Tripartite efflux pumps are essential for Gram-negative bacteria to expel a wide range of toxic compounds, including antibiotics, across their dual-membrane cell envelope. Among these systems, the AcrAB–TolC complex of *Escherichia coli* is one of the most thoroughly studied. It comprises the inner membrane RND (Resistance–Nodulation– Division) transporter AcrB, the periplasmic membrane fusion protein AcrA, and the outer membrane channel TolC. Structural analysis reveals that YbjP, a previously uncharacterized lipoprotein, binds TolC in a 3:3 stoichiometry, bridging its protomers at the equatorial domain.

Cryo-EM density reveals six AcrA molecules beneath each TolC trimer ([Fig fig2]), yielding a 3:6:3 stoichiometry for TolC:AcrA:AcrB. AcrA therefore forms an elongated hexamer that bridges TolC and AcrB. The trimeric TolC, which contains six HTH motifs due to internal repeats (TolC repeat 1/2), engages the AcrA hexamer via quasi-equivalent binding: adjacent AcrA and AcrA* protomers interact differentially with the intra- and inter-protomer grooves of TolC, respectively ([Fig fig2]). Upon engagement with AcrA’s α-helical hairpin domain, TolC helices rotate outward in a left-handed (counterclockwise) manner to open the channel, and enables small-molecule substrates to be exported through the fully assembled complex. A comparative structural analysis of TolC in its closed and open states reveals a striking iris-like dilation mechanism at the periplasmic entrance that facilitates transition to the fully open conformation ([Fig fig3]). Throughout this conformational transition, the transmembrane β-barrel and α-helical barrel domains maintain remarkable structural rigidity, whereas the coiled-coil helices undergo dramatic rearrangement. These helices pivot around the equatorial domain, undergoing a 27° rigid-body superhelical rotation ([Fig fig3]), which constitutes a major structural rearrangement. Notably, YbjP remains stably association with TolC in both conformational states – the closed resting state and the open activated state ([Fig fig3]). This persistent interaction suggests that YbjP serves as a structural scaffold: anchoring TolC in the outer membrane, accommodating conformational changes during activation, and functionally compensating for TolC’s lack of intrinsic lipidation.

>[6x]MNKNRGFTPLAVVLMLSGSLALTGCDDKQAQQGGQQMPAVGVVTVKTEPLQITTELPGRTSAYRIAEVRPQVSGIILKRNFKEGSDIEAGVSLYQIDPATYQATYDSAKGDLAKAQAAANIAQLTVNRYQKLLGTQYISKQEYDQALADAQQANAAVTAAKAAVETARINLAYTKVTSPISGRIGKSNVTEGALVQNGQATALATVQQLDPIYVDVTQSSNDFLRLKQELANGTLKQENGKAKVSLITSDGIKFPQDGTLEFSDVTVDQTTGSITLRAIFPNPDHTLLPGMFVRARLEEGLNPNAILVPQQGVTRTPRGDATVLVVGADDKVETRPIVASQAIGDKWLVTEGLKAGDRVVISGLQKVRPGVQVKAQEVTADNNQQAASGAQPEQSKS;>MKKLLPILIGLSLSGFSSLSQAENLMQVYQQARLSNPELRKSAADRDAAFEKINEARSPLLPQLGLGADYTYSNGYRDANGINSNATSASLQLTQSIFDMSKWRALTLQEKAAGIQDVTYQTDQQTLILNTATAYFNVLNAIDVLSYTQAQKEAIYRQLDQTTQRFNVGLVAITDVQNARAQYDTVLANEVTARNNLDNAVEQLRQITGNYYPELAALNVENFKTDKPQPVNALLKEAEKRNLSLLQARLSQDLAREQIRQAQDGHLPTLDLTASTGISDTSYSGSKTRGAAGTQYDDSNMGQNKVGLSFSLPIYQGGMVNSQVKQAQYNFVGASEQLESAHRSVVQTVRSSFNNINASISSINAYKQAVVSAQSSLDAMEAGYSVGTRTIVDVLDATTTLYNAKQELANARYNYLINQLNIKSALGTLNEQDLLALNNALSKPVSTNPENVAPQTPEQNAIADGYAPDSPAPVVQQTSARTTTSNGHNPFRN[3x];>MRYSKLTMLIPCALLLSACTTVTPAYKDNGTRSGPCVEGGPDNVAQQFYDYRILHRSNDITALRPYLSDKLATLLSDASRDNNHRELLTNDPFSSRTTLPDSAHVASASTIPNRDARNIPLRVDLKQGDQGWQDEVLMIQEGQCWVIDDVRYLGGSVHATAGTLRQSIENR[3x]>[2x]MVLYFIGLGLYDERDITVKGLEIAKKCDYVFAEFYTSLMAGTTLGRIQKLIGKEIRVLSREDVELNFENIVLPLAKEN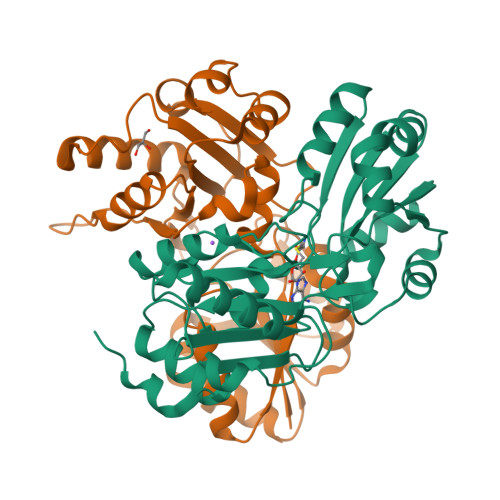DVAFLTPGDPLVATTHAELRIRAKRAGVESYVIHAPSIYSAVGITGLHIYKFGKSATVAYPEGNWFPTSYYDVIKENAERGMHTLLFLDIKAEKRMYMTANEAMELLLKVEDMKKGGVFTDDTLVVVLARAGSLNPTIRAGYVKDLIREDFGDPPHILIVPGKLHIVEAEYLVEIAGAPREILRVNV6-(trifluoromethyl)-3-{[4-(trifluoromethyl)benzyl]amino}quinoxaline-2-carboxylic acid | C18 H11 F6 N3 O2 | 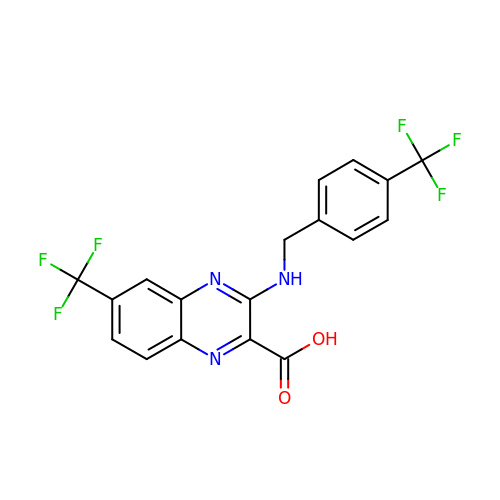FEJSMMIZTOMLEL-UHFFFAOYSA-N> DRHHHHHH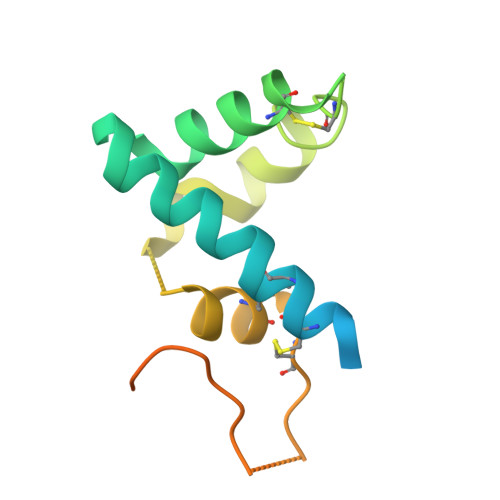KLSRAHDNQPGTIRSDHYTCVGCVLVVSVIEQLAQVHNSTVQASMERLCSYLPEEWVLKTACYMMVHVFGADIIKLFDKDVNADVVCHTLEFCKQEPGQPLCHLYPLPKESWKFTLEKARHIVKQSPIMKYTR> NNPYLFRSNKFLTLFKNQHGSLRLLQRFNEDTEKLENLRDYRVLEYCSKPNTLLLPHHSDSDLLVLVLEGQAILVLVNPDGRDTYKLDQGDAIKIQAGTPFYLINPDNNQNLR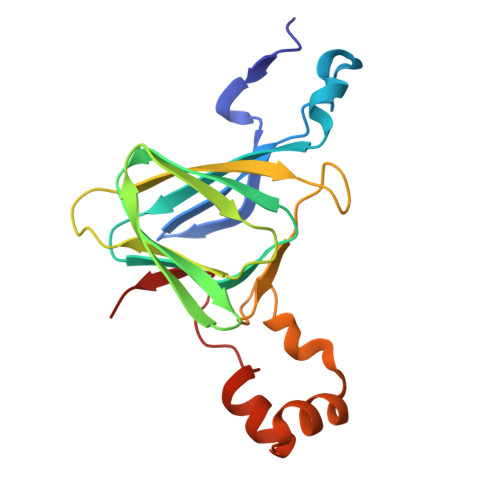ILKFAITFRRPGTVEDFFLSSTKRLPSYLSAFSKNFLEASYDSPYDEIEQTLLQEEQEGVIVKMP> MSHHHHHHSMRPSLSDYQHVASGKVRELYRVDDEHLLFVATDRISAFDFVLDTPIPDKGRILTAMSVFFFGLLTVPNHLAGPPDDPRIPEEVLGRALLVRRLDMLPVECVARGYLTGSGLLDYQRTGAVCGHVLPQGLGEASRLDPPLFTPATKADIGEHDMNVDFAAVVGLVGAVRANQLRDETIKIYTRAAAHALHKGIILADTKFEFGVDIEGNLVLADEVFTPDSSRYWDAAHYQPGVVQDSFDKQFVRNWLTGPESGWDRASDTPPPPLPDEVAVA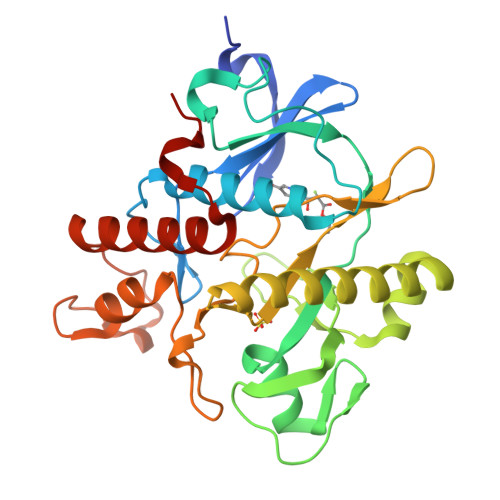TRERYIEAYERISGLSFSDWIGPSA>GPAMSYRVSTGAAHAAKGGGLVSGDSYSMMELGARKYAAAISDGMGNGARAHFESNETIKLLEKILESGIDEKIAIKTINSILSLRTTDEIYSTLDLSIIDLQDASCKFLKVGSTPSFIKRGDQVMKVQASNLPIGIINEFDVEVVSEQLKAGDLLIMMSDGIFEGPKHVENHDLWMKRKMKGLKTNDPQEIADLLMEEVIRTRSGQIEDDMTVVVVRIDHNT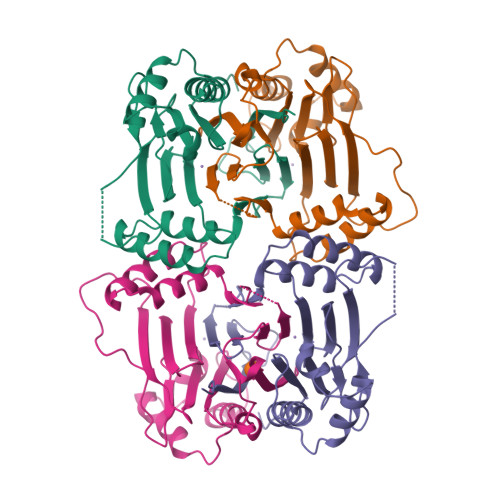PKWASIPVPAIFQNKQEIS[2x]>[20x]MKYVVVSGGVISGIGKGVLASSTGMLLKTLGLKVTSIKIDPYMNIDAGTMSPLEHGECFVLDDGGETDLDLGNYERYLGITLSRDHNITTGKIYSHVISRERRGDYLGKTVQIVPHLTNAIQDWIQRVSKIPVDDTGLEPDVCIIELGGTVGDIESAPFVEALRQFQFEVGRENFALIHVSLVPVIHGEQKTKPTQAAIKDLRSLGLIPDMIACRCSEELNRSTIDKIAMFCHVGPEQVVNVHDVNSTYHVPLLLLKQHMIDYLHSRLKLGEVPLTLEDKERGSQLLTNWENMTKNLDDSDDVVKIALVGKYTNLKDSYLSVTKSLEHASMKCRRQLEILWVEASNLEPETQEVDKNKFHDSWNKLSSADGILVPGGFGTRGIEGMILAAKWARESGVPFLGVCLGLQVAAIEFARNVIGRPNSSSTEFLDETLLAPEDQVVITMRLGLRPTIFQPNSEWSNIRKLYGEVNEVHERHRHRYEINPKIVNDMESRGFIFVGKDETGQRCEIFELKGHPYYVGTQYHPEYTSKVLEPSRPFWGLVAAASGTLGEVIKDINL

CTP synthase (CTPS) catalyzes the final, rate-limiting step of de novo CTP biosynthesis (Lieberman, 1956). Each CTPS monomer consists of a glutaminase domain and an amido-ligase domain connected by an alpha helical linker. Glutamine hydrolysis in the glutaminase domain produces ammonia which is transferred through a channel into the amido-ligase domain, where it is ligated to UTP to form CTP in an ATP-dependent process. Budding yeast have two CTPS isoforms, Ura7 and Ura8, which share 78 % identical residues.

We determined structures of CTPS filament bundles formed at pH 6.0 to better understand the mechanisms of lateral assembly. Reference-free two-dimensional averages of bundle segments from cryo-EM images of Ura7 and Ura8 were strikingly regular, suggesting ordered assembly contacts. This high degree of order allowed us to determine three-dimensional structures of both homologs in the presence of substrates or product using a single particle reconstruction approach by focused refinement of interacting pairs of filaments. As we found for the single filament structures, Ura8 reconstructions went to higher resolution (3.3 Å for substrates and 3.7 Å for product) than Ura7 (6.6 Å substrate and 7.0 Å product). The Ura8 substrate-bound structure had the same architecture as both Ura7 bundles, but the product-bound Ura8 structure had very different interfaces between filaments, giving rise to filaments in register. To better understand the nature of lateral assembly contacts, we built atomic models into the two Ura8 bundle structures. Ligands were clearly visible, and bound as in the single filament structures, and the longitudinal assembly interfaces were the same as observed in the single filaments. Domain rotations and the state of the closed ammonia channel were nearly identical between filaments and bundles. Unlike single Ura8 filaments determined at an intermediate pH (6.5) and with two rotamers for His360, the bundle map appeared to fit a single rotamer which points to D370. Yeast CTPS has a 7-residue insert (residues 273–279) in the linker region that mediates the bulk of the lateral interaction in both bundle types. In the substrate-bound structure, Leu277 nestles into a hydrophobic pocket formed by Ile383/Ile387/Ile412/Phe429.>[2x]SSQRSVARMDGDVIIGALFSVHHQPPAEKVPERKCGEIREQYGIQRVEAMFHTLDKINADPVLLPNITLGSEIRDSCWHSSVALEQSIEFIRDSLISIRDEKDGLNRCLPDGQTLPPGRTKKPIAGVIGPGSSSVAIQVQNLLQLFDIPQIAYSATSIDLSDKTLYKYFLRVVPSDTLQARAMLDIVKRYNWTY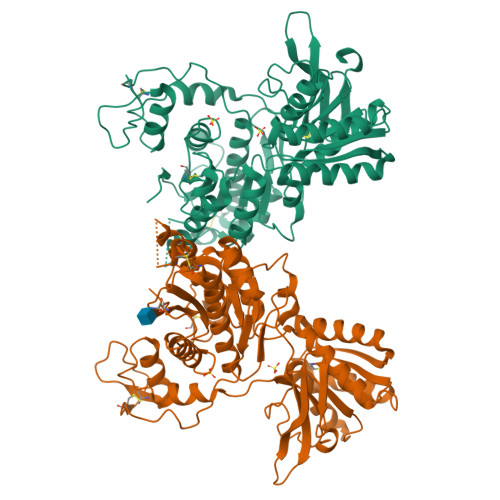VSAVHTEGNYGESGMDAFKELAAQEGLCIAHSDKIYSNAGEKSFDRLLRKLRERLPKARVVVCFCEGMTVRGLLSAMRRLGVVGEFSLIGSDGWADRDEVIEGYEVEANGGITIKLQSPEVRSFDDYFLKLRLDTNTRNPWFPEFWQHRFQCRLPGHLLENPNFKKVCTGNESLEENYVQDSKMGFVINAIYAMAHGLQNMHHALCPGHVGLCDAMKPIDGRKLLDFLIKSSFVGVSGEEVWFDEKGDAPGRYDIMNLQYTEANRYDYVHVGTWHEGVLNIDDYKIQMNKSGMVRS> MASMTGGQQMGMPAITCVWSDGRSDTWPNVNGHSRTRSVPSLKPLPHQDSKNLLYRQICGRLLAQHVFGGAGSTQPILNQLCKRLSTGNPNNTNASTVVTAPEKNVVSARHVRPNPKSSKDTLEKQPKYSSQIYLTDSFENYYLASLPTNYQLYQRDSNRENGNGKREFWLYGHPSGRPFRSVND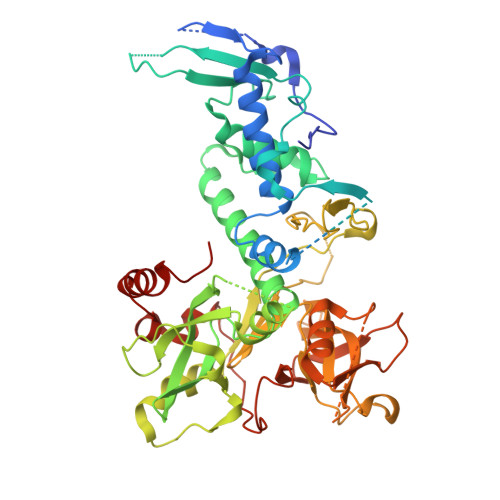FLHHLYWLISDLTRNESTCCCVLCSGNMTRVRKNLQKENERMFHECKDDTYTWPSSYRLGEVVWIDINNELIPAIIVARNLINYESNQMDAVKLISDTFVEPYQYHCKQLGNSRYYFDMAAADIEPWSRHPLDLQKQEHLVAHSICQTWNLFGIFQPLEGIDMEEPKFHDENYSIPLTVLPTFGGESNSLDDHFYGIFRGAEKLWINDLCVISTSSLPSVLQKTSFMYISDIYVNEDDIVCFQGSLWTQIDKNALDYNDSADNIDEHKDDLKELPRRLQMVSKLSNTYFRCLHDKSVEYVCPFADVLGRWYEPWFVKGDLNYTSEVKERTSSRLSAVGSENWVDDDFYEYLLSEIDMVSAVVM>[8x]ATRTRGYVTTKDGIKWYYEQEGSGPDVVLIPDGLGECQMFDKPMSLIASNGFRVTTFDMPGMSRSSDAPPETYQDITGRKLAGYIITLLDTLDIKIASVWGCASGASTVLALCSDYPERVRNGMPHEVPTENPDILLHIHEVDPATISQEMAANSRAASGNVEAWD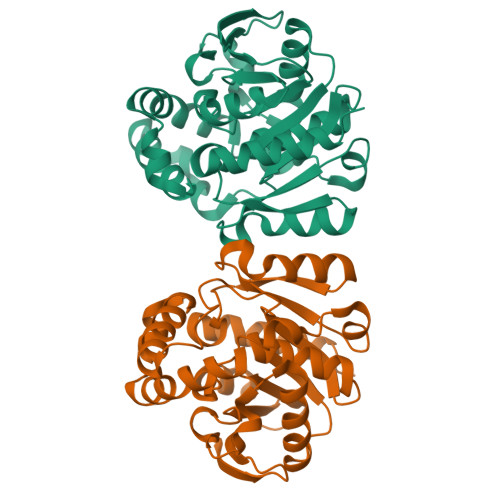ALGPEVHARLHDNYPRWAYGYPRTIPPSAPVKTEDLHKVPIDWTVGASTPTKLFFENIVIAAREGINIGTLPGNHFPYVSHPEEFAKYVVETSRKYLK>[3x]MEMLTKFESRSSRAAGVAFHPTQPWILTSLHNGRIQLWDYRMGTLLDRFDGHDGPVRGIAFHPTQPLFVSGGDDYKVNVWNYKSRKLLFSLCGHMDYVRVCTFHHEYPWILSCSDDQTIRIWNWQSRNCIAILTGHSHYVMCAAFHPSEDLIVSASLDQTVRVWDISGLRMKNAAPVSMSKEDQKAQAHNSKSNDKKGSTDAIVKFVLEGHDRGVNWCAFHPTLPLILSAGDDRLVKLWRMT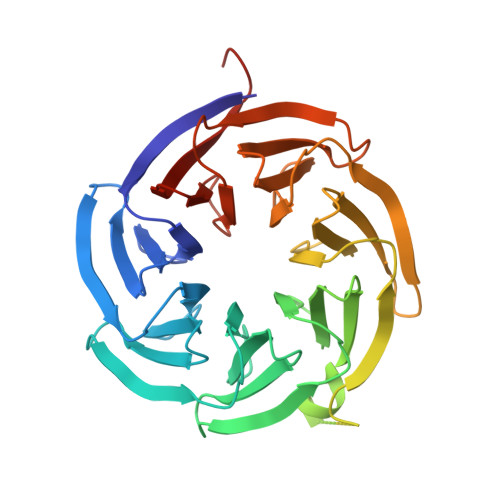ASKAWEVDTCRGHFNNVSCCLFHPHQELILSASEDKTIRVWDLNRRTAVQTFRRDNDRFWFITVHPKLNLFAAAHDSGVMVFKLESAWSHPQFEK The structure of the N-sites of HIV-1 RT and HBV Pol are considered to be quite similar, as the amino acid sequences that form the N-sites (referred to as motifs A, B, C, D, and E) are moderately conserved in both. In our previous studies, we examined various combinations of amino acid substitutions in motifs A–E and found that the HBV-RT-associated 3MB mutant comprising Q151M in motif B and Y115F/F116Y in motif A is useful as a surrogate for structurally studying HBV RT since HIV-1 harboring RT3MB turned out to be highly sensitive against typical anti-HBV NAs, ETV, and 3TC. E-CFCP is a 4′-modified and fluoromethylenated NA that exhibits potent antiviral activity against both wild-type and drug-resistant HBVs but less potent against human immunodeficiency virus type-1 (HIV-1). The present study aimed to elucidate the mechanism of potent antiviral activity of E-CFCP against wild-type and drug-resistant HBV using HIV-1 with HBV-associated mutations in RT.

We also determined the structures of HIV-1 RT4M complexed with DNA:ETV-TP/dGTP at 2.32 and 2.30 Å resolutions, respectively, as reference models for comparison. In contrast, the bound ETV-TP/dGTP are well ordered and superimposed with each other with an RMSD of 0.2–0.3 Å, and their average B-values were similar to those of polypeptide chains and DNA (~ 60 Å2), suggesting that the bound ETV-TP/dGTP is rather static within the N-site. ETV-TP has no 4′-modification but has an exocyclic methylene that pushes the Met184 sidechain backward. The results confirmed that RT4M is more susceptible to E-CFCP-TP compared to RTWT.

>[2x]MVPISPIETVPVKLKPGMDGPKVKQWPLTEEKIKALVEICTEMEKEGKISKIGPENPYNTPVFAIKKKDSTKWRKVVDFRELNKRTQDFWEVQLGIPHPAGLKQKKSVTVLDVGDAFYSVPLDKDFRKYTAFTIPSINNETPGIRYQYNVLPMGWKGSPAIFQSSMTKILEPFRKQNPDIVIYQYMDDLYVGSDLEIGQHRTKIEELRQHLLRWGFTTPDKKHQKEPPFLWMGYELHPDKWTVQPIVLPEKDSWTVNDIQKLVGKLNWASQIYAGIKVRQLSKLLRGTKALTEVVPLTEEAELELAENREILKEPVHGVYYDPSKDLIAEIQKQGQGQWTYQIYQEPFKNLKTGKYARMKGAHTNDVKQLTEAVQKIATESIVIWGKTPKFKLPIQKETWEAWWTEYWQATWIPEWEFVNTPPLVKLWYQLEKEPIIGAETFYVDGAANRETKLGKAGYVTDRGRQKVVPLTDTTNQKTELQAIHLALQDSGLEVNIVTDSQYALGIIQAQPDKSESELVSQIIEQLIKKEKVYLAWVPAHKGIGGNEQVDKLVSAG;>MAHHHHHHALEVLFQGPISPIETVPVKLKPGMDGPKVKQWPLTEEKIKALVEICTEMEKEGKISKIGPENPYNTPVFAIKKKDSTKWRKLVDFRELNKRTQDFWEVQLGIPHPAGLKQKKSVTVLDVGDAYFSVPLDKDFRKYTAFTIPSINNETPGIRYQYNVLPQGWKGSPAIFQSSMTKILEPFRKQNPDIVIYQYMDDLYVGSDLEIGQHRTKIEELRQHLLRWGFTTPDKKHQKEPPFLWMGYELHPDKWTVQPIVLPEKDSWTVNDIQKLVGKLNWASQIYAGIKVRQLSKLLRGTKALTEVVPLTEEAELELAENREILKEPVHGVYYDPSKDLIAEIQKQGQGQWTYQIYQEPFKNLKTGKYARMKGAHTNDVKQLTEAVQKIATESIVIWGKTPKFKLPIQKETWEAWWTEYWQATWIPEWEFVNTPPLVKLWYQ[2x]>GANAYLNLYKIDIPKKIKRLYFYNPDMEPKLFARNLSRVNNFKFQDSNDLVWIEIPDIDFQITPKNVFQYKVEKEEIIKEEEDKKLFVKTLYKYIKKLFLDNDFYFKKGNNFISNSEVFSLDSNENVNAHLTYKIKIHNISNEYYLSILPKFTFLSKEPALESAIKSGYLYNIKSGKSFPYISGLDGILKIDIGNNQIVEVAYPENYLFNFTTRDAEKYGFSKEVHEIYKNKVFEGFKKIPKTLGFLNKITNLNENYQLKDGYKIFINVIYKFKNGESRYAKDVFKYSFYKNEQPLKAIFFFSSKKQFFEVQKSLKELFHNKHSVFYRAAAELGFSKVEFLRDSKTKSSAFLYNPEEFTVKNTEFINQIEDNVMAIVLLDKYIGNIDPLVRNFPDNLILQPILKEKLEDIKPFIIKSYVYKMGNFIPECKPFILKKMEDKEKNLYIGIDLSHDTYARKTNLCIAAVDNTGDILYIGKHKNLELNEKMNLDILEKEYIKAFEKYIEKFNVSPENVFILRAGRFIEDIEIIKNFISYNDTKYTLVEVNKNTNINSYDDLKEWIIKLDENTYIYYPKTFLNQKGVEVKILENNTDYTIEEIIEQIYLLTRVAHSTPYTNYKLPYPLHIANKVALTDYEWKLYIPY[2x]

Argonaute (Ago) proteins exist in all three domains of life. The N-terminal and PIWI-Argonaute-Zwille (PAZ) domains constitute the amino-terminal lobe (N-lobe), while the middle (MID) and the catalytic RNase H-like P element-induced wimpy testis (PIWI) domains form the carboxyl-terminal lobe (C-lobe). Unlike other Argonautes, the Ago protein from the eubacterium Marinitoga piezophila (MpAgo) has been shown to preferentially bind 5′-hydroxylated guide RNAs to target ssDNA. Here we present a crystal structure of MpAgo bound to an RNA guide sequence and a complementary DNA target strand, providing insight into preferential targeting of ssDNA.

In order to capture a target-bound structure, we mutated an aspartate residue to an alanine (D516A) in the enzyme’s catalytic pocket to prevent DNA cleavage. Nucleotides 1–20 of the guide RNA (orange) and 2–21 of the target DNA (red) are ordered with a straight helical axis passing through the central cleft of the protein. The heteroduplex bound by MpAgo contains more ordered nucleotides, with 20 base pairs modeled within the duplex, than previously crystallized Ago complexes. Recognition and subsequent binding of the DNA target results in movement of the N-lobe away from the C-lobe to accommodate the hybrid helix. The MpAgo ternary complex shows that the 5′ nucleotide of the guide remains bound to the MID domain and unpaired to the 3′ terminal nucleotide C21 of the DNA target. The insertion of F410 between C20 and C21 disrupts the helical base stacking, splaying the terminal base away from the hybrid helix, while K279 of Linker L2 interacts with the phosphate backbone to stabilize the contorted 3′ end of the DNA target. The MpAgo ternary structure shows that ß-strands 1 and 2 twist away from ß-strand 3 to create a path for the glutamate finger to complete the catalytic tetrad. The geometry of the heteroduplex within the MpAgo ternary complex aligns more closely with a perfect B-form helix instead of an A-form helix. The 5′ region of the MpAgo DNA target (positions 5–8) interacts through the phosphate backbone with charged residues (K93, K107, and K174) positioned at the interface of Linker L1 and the PAZ and N-terminal domains. In contrast, the N-terminal domain of MpAgo does not split the guide and target strands, but instead the helix remains intact through the central channel of the protein.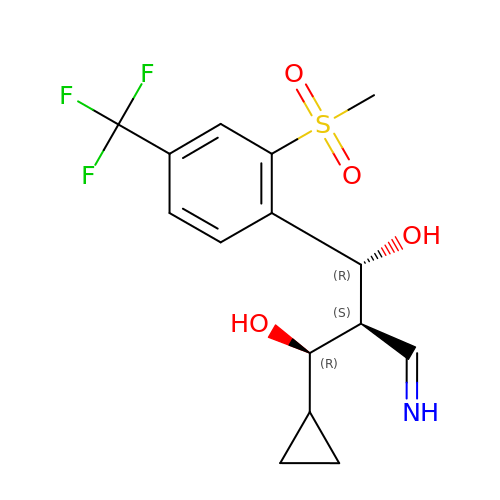(1R,2S,3R)-1-cyclopropyl-2-(iminomethyl)-3-[2-methylsulfonyl-4-(trifluoromethyl)phenyl]propane-1,3-diol | C15 H18 F3 N O4 S | GOAAJVFYZPNLHO-MAVPCDBQSA-N>MDARTSIEQRSNAVSQVLLGIFSYVRWPKEP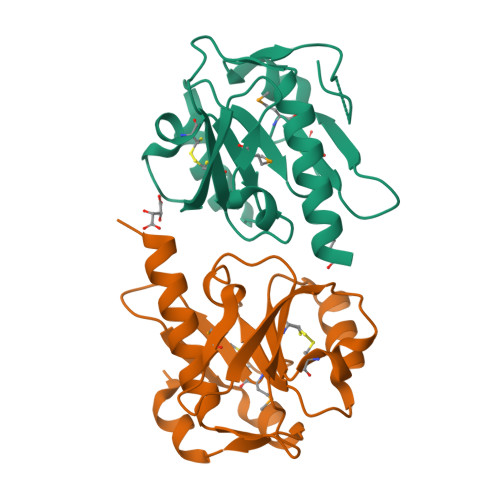AVLQLCVVGPTEYADGLLRGMVQANGRRVHAERRAVDNPDLGTLCNVIYLGVVDERERQQVFRSLAGHPVLSISERGTECSVGSMFCLNVGGPRITFEANLDSIARSGVRVHPSVLKLARRQATPLEHHHHHH[4x]> YDGQNCKEPGNCWENKPGYPEKIAGSKYDPKHDPVE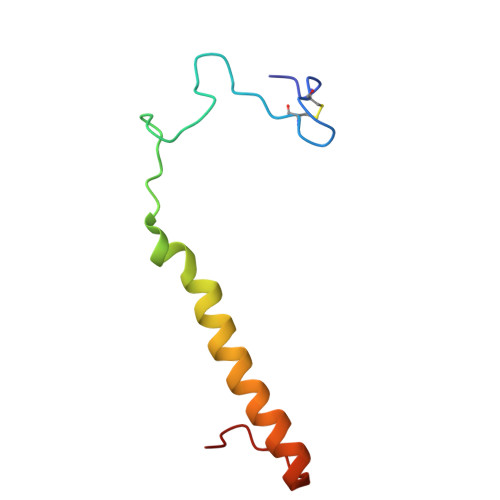LNKQEESIKAMDARNAKRIANAKSSGNFVFDVK> MTMADETIILNVLGQYTRAHDRRDPDAM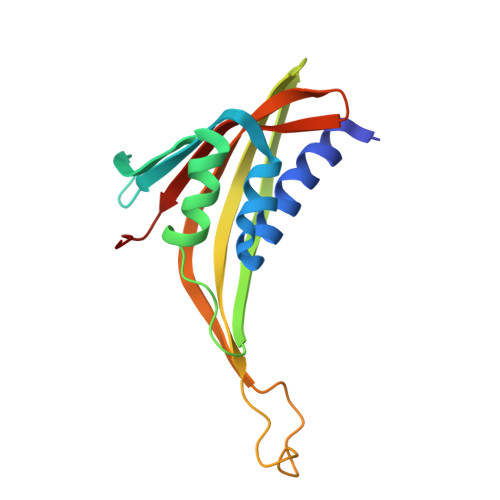AALFAPDASIVVLDAVGGASKPISVLHGRDAIRVAVRQMMAPHGYRAWSQNVVNAPVIHIHGDTARLDAQFMVFSILAAEVPDGGWPTGTFGAQGRIVPIEAGTYTLFLRTVPDGWVIAHMVIKHRLPMAFG A third vital component of the TFP biogenesis system is the assembly ATPase (PilF in T. thermophilus). The TFP assembly ATPases are part of the extensive AAA+ superfamily which form molecular motors, using the energy from ATP hydrolysis to drive mechanical transformations. The domain structure of T2SS and TFP biogenesis ATPases is similar, in that they comprise one or more N1 or GSPII domains at the N-terminus, followed by a C-terminal (CTD) and N2 domain- which comprise the ATP binding site. Here we present a combination of X-ray crystallographic and cryoelectron microscopy single particle reconstructions of the PilF hexamer in two states which are used to build molecular models for the complete PilF hexamer and chart its structural transition on binding of ATP.

Crystallization trials on the complete TtPilF hexamer were unsuccessful; however, limited proteolysis gave rise to a fragment of approximate molecular mass 44 kDa which was purified and yielded crystals which diffracted to 2.44 Å. Mass spectrometry was used to confirm that this fragment corresponded to the C-terminal half of the protein, encompassing the N2, CTD and Zn-binding domains (designated TtPilFc). TtPilFc forms a flattened hexamer, with 2-fold rotational non-crystallographic symmetry relating the two trimers. Inspection of all 6 binding sites revealed electron density consistent with bound nucleotide; however, there was no evidence for ATP hydrolysis in any site. ATPase assays were carried out on the TtPilFc fragment which showed that it was not enzymatically active, confirming that the fragment is catalytically inert in solution, as well as in the crystalline state. Thr651, Gly652, Ser653, Lys655 and Ser656 form part of the Walker A motif involved in binding the γ and β phosphates. One possible explanation for the failure of the TtPilFc fragment to hydrolyse ATP is the conformation of the linker polypeptide between the CTD and N2 domains. Significant differences were apparent between the TtPilFAMPPNP model and the TtPilFc crystal structure. Superposition of the CTD and N2 domains gave an r.m.s. displacement of 3.47 Å for Cα atoms; when viewed from the top, TtPilFc is wider by about 6 Å along the long axis and shorter by 7 Å along the shorter axis, leading to a flatter hexagonal shape. We find that TtPilFc is wider and flatter than its equivalent density in the complete hexamer in the AMPPNP-bound state, indicating that the presence of the N1 domains does affect the relative orientations of the ATPase domains.

>[6x]LELDESAAQKFVKQVIREAFLQDASDIHIEPRQNDVQVRLRIDGALRPYSTLPKGALNAVISVVKIMGGLNIAEKRLPQDGRVRYREGAIDVDLRLSTLPTVYGEKAVMRLLKKASDIPEIEDLGFAPGVFERFKEVISKPYGIFLITGPTGSGKSFTTFSILKRIATPDKNTQTIEDPVEYEIPGINQTQVNPQAGLTFARALRAFLRQDPDIIMVGEIRDSETAKIATEAALTGHLVIATLHTNDAAQAITRLDEMGVEPFNISAALIGVLSQRLVRRVCEHCKVEVKPDPETLRRLGLSEAEIQGARLYKGMGCERCGGTGYKGRYAIHELLVVDDEIRHAIVAGKSATEIKEIARRKGMKTLREDGLYKALQGITTLEEVLARTIE>SNASASSIEKGQNRVIDASLTLIRERAKLKGELVRLLGGAKASTSLLGVPLGHNSSFLQGPAFAPPRIREAIWCGSTNSATEEGKELKDPRVLTDVGDVPVQEIRDCGVDDDRLMNVISESVKLVMEEEPLRPLVLGGDHSISYPVVRAVSEKLGGPVDILHLDAHPDIYDCFEGNKYSHASSFARIMEGGYARRLLQVGIRSINQEGREQGKRFGVEQYEMRTFSKDRPMLENLKLGEGVKGVYISIDVDCLDP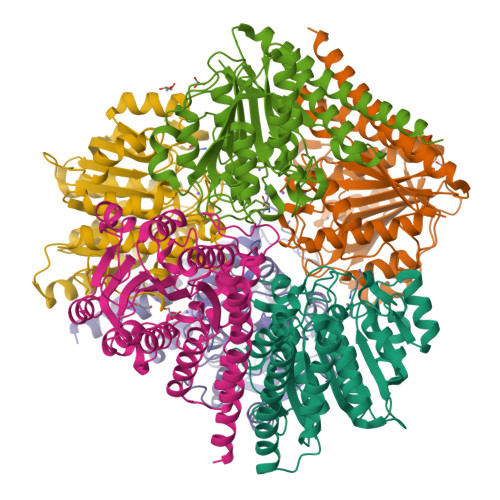AFAPGVSHIEPGGLSFRDVLNILHNLQADVVGADVVEFNPQRDTVDGMTAMVAAKLVRELAAKISK[24x]>QAQITGRPEWIWLALGTALMGLGTLYFLVKGMGVSDPDAKKFYAITTLVPAIAFTMYLSMLLGYGLTMVPFGGEQNPIYWARYADWLFTAPLLLLDLALLVDADQGTILALVGAAGIMIGTGLVGALTKVYSYRFVWWAISTAAMLYILYVLFFGFTSKAESMRPEVASTFKVLRNVTVVLWSAYPVVWLIGSEGAGIVPLNIETLLFMVLDVSAKVGFGLI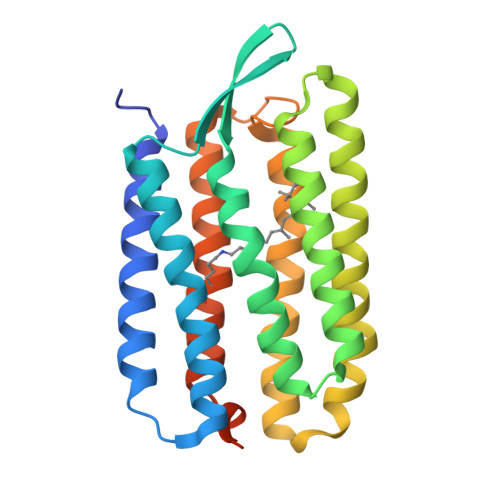LLRSRAIFGEAEAPEPSAGDGAAATSD[2x]> VCPNIIKRSAWEARETHCPKMNLPAKYVIIIHTAGTSCTVSTDCQTVVRNIQSFHMDTRNFCDIGYHFLVGQDGG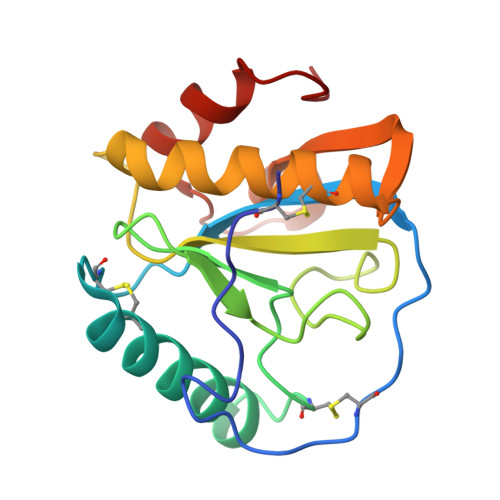VYEGVGWHIQGSHTYGFNDIALGIAFIGYFVEKPPNAAALEAAQDLIQCAVVEGYLTPNYLLMGHSDVVNILSPGQALYNIISTWPHFKH>[2x]MASATFTGVIPPVMTPLHADGSVDVESLRKLVDHLINGGVDGLFALGSSGEAAFLTRAQRKLALTTIIEHTAGRVPVTAGVIETTTARVIELVEDALEAGAEGLVATAPFYTRTHDVEIEEHFRKIHAAAPELPLFAFNIPVSVHSNLNPVMLLTLAKDGVLAGTKDSSGNDGAIRSLIEARDDAGLTEQFKILTGSETTVDFAYLAGA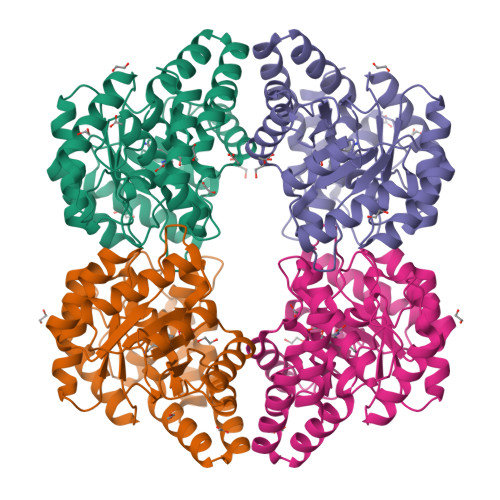DGVVPGLGNVDPAAYAALAKLCLDGKWAEAAALQKRINHLFHIVFVGDTSHMSGSSAGLGGFKTALAHLGIIESNAMAVPHQSLSDEETARIHAIVDEFLYTA Cytochromes c' are soluble periplasmic heme proteins widely distributed among Gram-negative bacteria from psychrophiles to thermophiles. The vast majority of cytochromes c' consist of homodimeric subunits with each monomer forming either a four-α helix bundle or a β sheet structure, called cytochrome c'-α or cytochrome c'-β, respectively. Both types of cytochromes c' contain a penta-coordinate heme per subunit, in which the heme Fe binds to an endogenous conserved proximal His ligand and their distal sites are vacant. Cytochrome c' has an ability to bind diatomic gases such as nitric oxide (NO) through the heme in vitro, indicating possible cellular functions as NO sensor or scavenger.

Here, we characterize a thermally stable cytochrome c′-α from thermophilic Hydrogenophilus thermoluteolus (PhCP-α) to understand how protein thermal stability affects NO binding. To understand the structural reasons for the slow NO binding in PhCP-α, the crystal structure of NO-soaked Fe(II) PhCP-α was determined at 1.6 Å resolution in space group P6222, which was the same as that of the native Fe(III) PhCP-α crystal without NO. The NO-soaked Fe(II) PhCP-α structure differs from that of the native PhCP-α in that the proximal His-128 ligand was dissociated from the heme center, and instead electron density consistent with an NO molecule is observed at the proximal heme face with the NO N and heme Fe distance of 1.90 ± 0.15 Å and Fe-N-O angle of 105°. The N-Fe distances in AxCP-α and SfCP-α (for subunit A) are 1.73 ± 0.10 and 1.75 ± 0.07 Å, respectively, indicating no statistical difference in Fe-NO coordination lengths among PhCP-α, AxCP-α, and SfCP-α. In the heme proximal region of PhCP-α, Arg-75 forms a salt bridge with Glu-135 near the Arg-132 residue before and after the NO binding. This salt bridge formation may confer conformational rigidity to the heme proximal region. Although there is no favorable hydrogen-bonding geometry between the NO ligand and Arg-132 in PhCP-α, we note that the distance to the Nη atom (3.4 and 3.7 Å for the N and O atoms, respectively) is somewhat less than between NO and the Nη atom of Arg-124 in AxCP-α (4.2 and 4.0 Å for the N and O atoms, respectively). In native PhCP-α structure, the heme distal region is occupied by a bulky aromatic Tyr-16 residue that locates in parallel to the heme face, where it can sterically hinder heme-gas coordination and/or π-stack with the porphyrin ring to possibly change the electrochemical properties. Using structural and spectroscopic techniques, we show that the thermally stable cytochrome c' from Hydrogenophilus thermoluteolus exhibits slow heme-NO binding compared with mesophilic and psychrophilic counterparts, a difference that we attribute to conformational rigidity around the heme.

> ALKPEDKVKFRQASYTTMAWNMGKIKAMVVDGTMPFSQTQVSAAANVIAAIANSGMGALYSPDTLGVVGFKKSRLKENFFQEQDEVRKIATNFVEQANKLAEVAAMGDKDEIKAQFGEVGKACKACHEKFREEE>[2x]SEITLGKYLFERLKQVNVNTVFGLPGDFNLSLLDKIYEVEGMRWAGNANELNAAYAADGYARIKGMSCIITTFGVGELSALNGIAGSYAEHVGVLHVVGVPSISSQAKQLLLHHTLGNGDFTVFHRMSANISETTAMITDIATAPAEIDRCIRTTYVTQRPVYLGLPANLVDLNVPAKLLQTPIDMSLKPNDAESEKEVIDTILALVKDAKNPVILADACCSRHDVKAETKKLIDLTQFPAFVTPMGKGSISEQHPRYGGVYVGTLSKPEVKEAVESADLILSVGALLSDFNTGSFSYSYKTKNIVEFHSDHMKIRNATFPGVQMKFVLQKLLTNIADAAKGYKPVAVPARTPANAAVPASTPLKQEWMWNQLGNFLQEGDVVIAETGTSAFGINQTTFPNNTYGISQVLWGSIGFTTGATLGAAFAAEEIDPKKRVI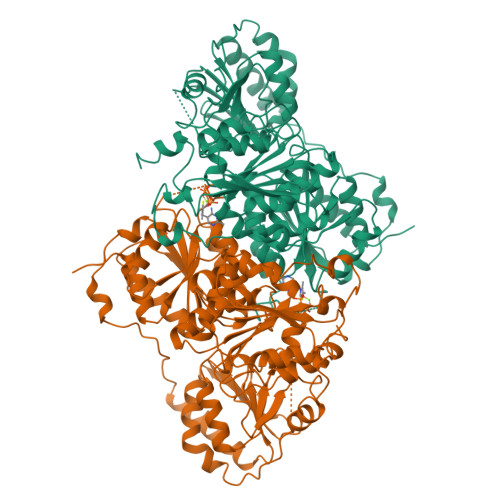LFIGDGSLQLTVQEISTMIRWGLKPYLFVLNNDGYTIEKLIHGPKAQYNEIQGWDHLSLLPTFGAKDYETHRVATTGEWDKLTQDKSFNDNSKIRMIEIMLPVFDAPQNLVKQAKLT> HHHATIKQRTLKNIIRATGVGLHSGEKVYLTLKPAPVDTGIVFCRTDLDPVVEIPARAENVGETTMSTTLVKGDVKVDTVEHLLSAMAGLGIDNAYVELSASEVPIMDGSAGPFVFLIQSAGLQEQEAAKKFIRIKREVSVEEGDKRAVFVPFDGFKVSFEIDFDHPVFRGRTQQASVDFSSTSFVKEVSRARTFGFMRDIEYLRSQNLA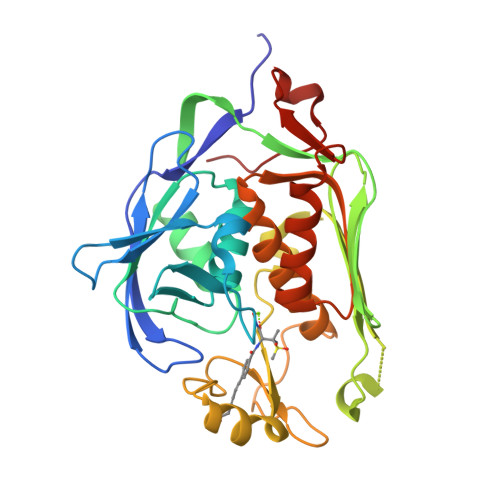LGGSVENAIVVDENRVLNEDGLRYEDEFVKHKILDAIGDLYLLGNSLIGEFRGFKSGHALNNQLLRTLIADKDAWEVVTFEDARTAPISYMRP> SDPENIKTQELFRKVRSILNKLTPQMFNQLMKQVSGLTVDTEERLKGVIDLVFEKAIDEPSFSVAYANMCRCLVTLKVPMADKPGNTVNFRK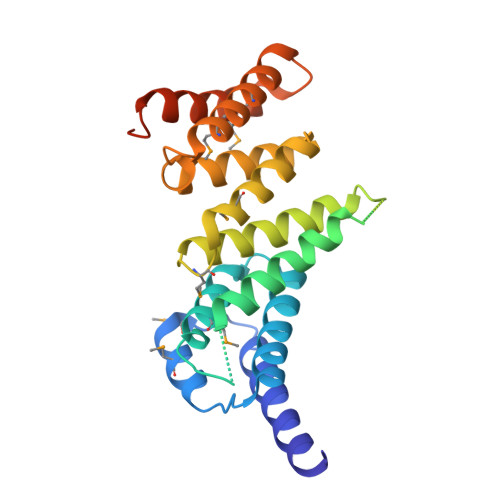LLLNRCQKEFEKDKADDDVFEKKQKELEAASAPEERTRLHDELEEAKDKARRRSIGNIKFIGELFKLKMLTEAIMHDCVVKLLKNHDEESLECLCRLLTTIGKDLDFEKAKPRMDQYFNQMEKIVKERKTSSRIRFMLQDVIDLRLCNWVSRRADQGPKTIEQIHKEA5-fluoro-2-({[(3M)-3-(4H-1,2,4-triazol-3-yl)pyridin-2-yl]amino}methyl)phenol 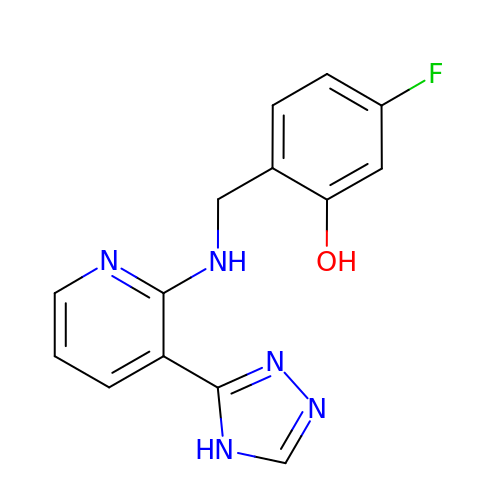| C14 H12 F N5 O | QRRUXNVQGIXBIR-UHFFFAOYSA-N> MGSSHHHHHHSQDPMSLNLVSEQLLAANGLKHQDLFAILGQLAERRLDYGDLYFQSSYHESWVLEDRIIKDGSYNIDQGVGVRAISGEKTGFAYADQISLLALEQSAQAARTIVRDSGDGKVQTLGAVEHSPLYTSVDPLQSMSREEKLDILRRVDKVAREADKRVQEVTASLSGVYELILVAATDGTLAADVRPLVRLSVSVLVEEDGKR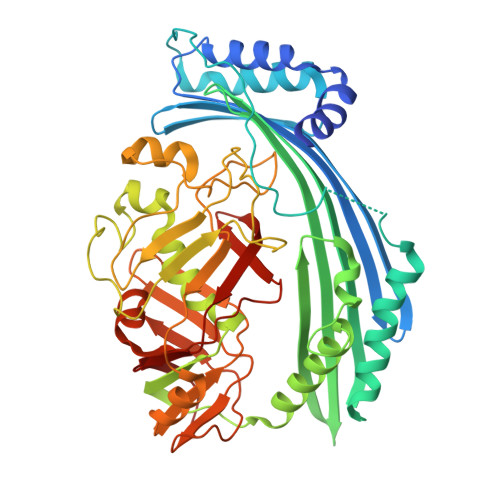ERGASGGGGRFGYEFFLADLDGEVRADAWAKEAVRMALVNLSAVAAPAGTMPVVLGAGWPGVLLAEAVGHGLEGDFNRRGTSVFSGQVGELVASELCTVVDDGTMVDRRGSVAIDDEGTPGQYNVLIENGILKGYMQDKLNARLMGMTPTGNGRRESYAHLPMPRMTNTYMLPGKSTPQEIIESVEYGIYAPNFGGGQVDITSDKFVFSTSEAYLIENGKVTKPVKGATLIGSGIETMQQISMVGNDLKLDNGVGVCGKEGQSLPVGVGQPTLKVDNLTVGGTA> GTLTGERPPVFWLQGQGCTGCSV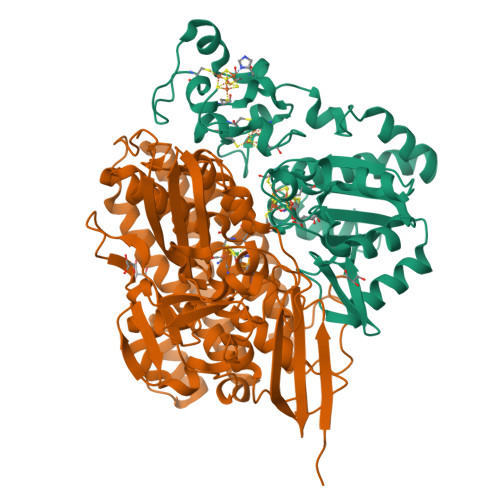TLLNSVHPSIADVLLKVISLEFHPTVMAWEGEHAIEHMRKVAEKFKGKFFLVIEGSVPVEADGKYCIIGEANHHEISMVDALKEFGPNAAAVLAVGTCAAYGGIPAAEGSETGATAVSKFLGDNGIKTPVVNIPGCPPHPDWIVGTVVLALDAIKKNGLEGGLAEVVKVLDSDGRPTPFFGRNIHENCPYLDKYDEGVMSATFTDKVGCRYDLGCKGPMTMADCFERKWNGGVNWCVQNAVCIGCVEPDFPDGKSPFYQA;> WSHPQFEKGATGRTTIAIDPVTRIEGHLKAEVVVENGKVVDARLSGTMYRGFETILRGRDPRDASQIVQRICGVCPTAHSTASVLALDEAFGAKVPNNGRITRNLIFGANYLQSHILHFYHLSAQDFVQGPDTAPFVPRFPKSDLRLSKELNKAGVDQYIEALEVRRICHEMVALFGGRMPHVQGQVVGGATEIPTKEKLVEYAARFKKVRDFVEQKYVPVVYTIGSKYKDMFKVGQGFKAALCVGAFPLDNSGKKHLFMPGVYAKGKDMPFDPSKIKEYVKYSWFAEETTGLNYKEGKTIPAPDKAGAYSFVKAPRYDGLSLEVGPLARMWVNNPELSPVGKKLLKDLFGISAKKFRDLGEEAAFSLMGRHVARAEETYYMLGAIEGWLKEIKAGEDTVVMPAVPASAEGTGFTEAPRGSLLHYVKVKDSKIDNYQIVSASLWNCNPRDDMGQRGAVEEALIGIPVDDIQNPVNVARLIRAFDPULGCAVH> TEMSVRKIAAHMKSNPNAKVIFMVGAGISTSCGIPDFRSP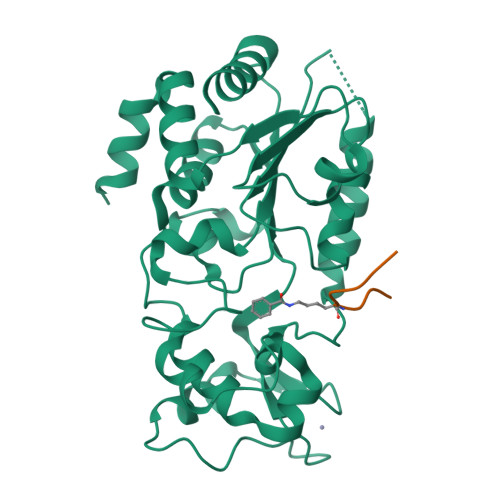GTGLYHNLARLKLPYPEAVFDVDFFQSDPLPFYTLAKELYPGNFRPSKFHYLLKLFQDKDVLKRVYTQNIDTLERQAGVKDDLIIEAHGSFAHCHCIGCGKVYPPQVFKSKLAEHPIKDFVKCDVCGELVKPAIVFFGEDLPDSFSETWLNDSEWLREKITTSGKHPQQPLVIVVGTSLAVYPFASLPEEIPRKVKRVLCNLETVGDFKANKRPTDLIVHQYSDEFAEQLVEELGWQEDFEKILTAQ;> QTARKSTGGK> DGLYLQVGAFANPDAAELLKAKLSGVTAAPVFISSVVRNQQILHRVRLGPIGSADEVSRTQDSIRVANLGQPTLVRPD

However, it is known that the sporulation-related repeat (SPOR) domains (Pfam 05036), ubiquitous in prokaryotes, play a central role in directing proteins to the septum by recognition of the unique septal PG (rather than recognition by other division proteins), which is enriched in denuded glycans, the PG devoid of peptide stems. Of all SPOR-domain-containing proteins, RlpA is the most highly conserved across bacterial species, which underscores its important physiological role in bacteria. It is predicted to have two domains, a catalytic “double-ψ β-barrel” domain (DPBB; Pfam 03330) and a C-terminal SPOR domain. In the present report, we disclose the X-ray structure of the SPOR domain of rare lipoprotein A (RlpA) from P. aeruginosa (SPOR-RlpA).

In order to characterize how the SPOR-RlpA domain interacts with denuded PG, we solved the X-ray structure of the complex with compound 1. Co-crystallization and soaking were both performed in parallel and resulted in two structures for the SPOR-RlpA:1 complex at near-atomic resolution (1.30 and 1.48 Å, respectively). The two structures are identical (rmsd of 0.16 Å for the 77 Cα atoms); the description provided herein is for the 1.30 Å resolution cocrystallization complex. The opposite face (convex face) of the SPOR domain does not present any of the features observed for compound 1 interaction, thus pointing to a single PG-binding site per SPOR domain, consistent with the mass spectrometric data. The high-resolution data for the SPOR-RlpA:1 complex allowed us to map all the amino acids and water molecules involved in glycan-chain recognition. (ii) Notwithstanding that all four saccharides interact with the protein, interactions are not evenly distributed among the four subsites. (v) Main-chain interactions are essential in PG stabilization by SPOR domains. (vi) hydrophobic interactions are observed with F274 and L307. In agreement with our mass-spectrometric experiments that clearly noted the absence of binding of compound 5 to the SPOR domain, the crystal structure of SPOR-RlpA:1 reveals that recognition of the carboxylate moieties of muramic acids at positions 1 and 3 is crucial.> AMADIGSEFGHRTLASTPALWASIPCPRSELRLDLVLPSGQSFRWREQSPAHWSGVLADQV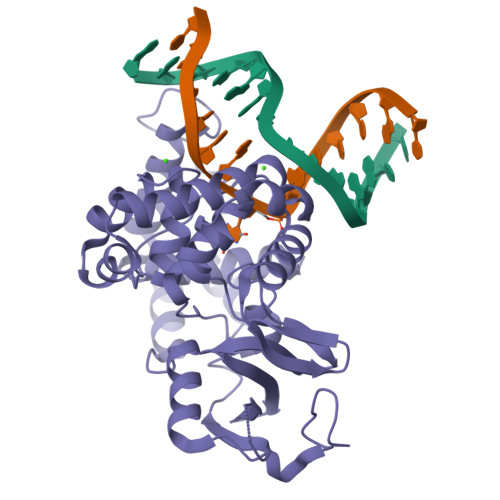WTLTQTEEQLHCTVYRGDKSQASRPTPDELEAVRKYFQLDVTLAQLYHHWGSVDSHFQEVAQKFQGVRLLRQDPIECLFSFICSSCNNIARITGMVERLCQAFGPRLIQLDDVTYHGFPSLQALAGPEVEAHLRKLGLGYRARYVSASARAILEEQGGLAWLQQLRESSYEEAHKALCILPGVGTQVADCICLMALDKPQAVPVDVAMWHIAQRDYSWHPTTSQAKGPSPQTNKELGNFFRSLWGPYAGWAQAVLFSADLRQSR>[2x]MNQNLLVTKRDGSTERINLDKIHRVLDWAAEGLHNVSISQVELRSHIQFYDGIKTSDIHETIIKAAADLISRDAPDYQYLAARLAIFHLRKKAYGQFEPPALYDHVVKMVEMGKYDNHLLEDYTEEEFKQMDTFIDHDRDMTFSYAAVKQLEGKYLVQNRVTGEIYESAQFLYILVA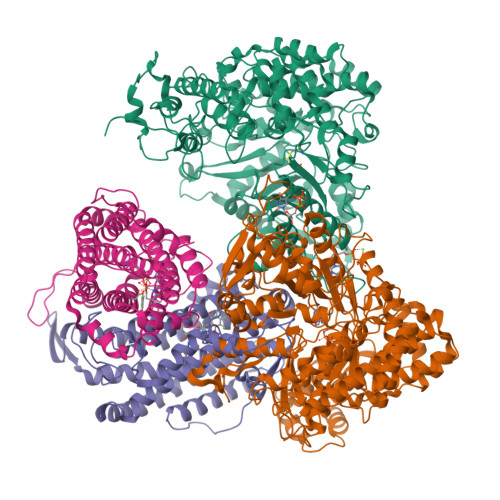ACLFSNYPRETRLQYVKRFYDAVSTFKISLPTPIMSGVRTPTRQFSSCVLIECGDSLDSINATSSAIVKYVSQRAGIGINAGRIRALGSPIRGGEAFHTGCIPFYKHFQTAVKSCSQGGVRGGAATLFYPMWHLEVESLLVLKNNRGVEGNRVRHMDYGVQINKLMYTRLLKGEDITLFSPSDVPGLYDAFFADQEEFERLYTKYEKDDSIRKQRVKAVELFSLMMQERASTGRIYIQNVDHCNTHSPFDPAIAPVRQSNLCLEIALPTKPLNDVNDENGEIALCTLSAFNLGAINNLDELEELAILAVRALDALLDYQDYPIPAAKRGAMGRRTLGIGVINFAYYLAKHGKRYSDGSANNLTHKTFEAIQYYLLKASNELAKEQGACPWFNETTYAKGILPIDTYKKDLDTIANEPLHYDWEALRESIKTHGLRNSTLSALMPSETSSQISNATNGIEPPRGYVSIKASKDGILRQVVPDYEHLHDAYELLWEMPGNDGYLQLVGIMQKFIDQSISANTNYDPSRFPSGKVPMQQLLKDLLTAYKFGVKTLYYQNTRDGAEDAQDDLVPSIQDDGCESGACKI;>[2x]MAYTTFSQTKNDQLKEPMFFGQPVNVARYDQQKYDIFEKLIEKQLSFFWRPEQVDVSRDRIDYQALPEHEKHIFISNLKYQTLLDSIQGRSPNVALLPLISIPELETWVETWAFSETIHSRSXTHIIRNIVNDPSVVFDDIVTNEQIQKRAEGISSYYDELIEMTSYWHLLGEGTHTVNGKTVTVSLRELKKKLYLCLMSVNALEAIRFYVSFACSFAFAERELMEGNAKIIRLIARDEALHLTGTQHMLNLLRSGADDPEMAEIAEECKQECYDLFVQAAQQEKDWADYLFRDGSMIGLNKDILCQYVEYITNIRMQAVGLDLPFQTRSNPIPWINTWLVSDNVQVAPQEVEVSSYLVGQIDSEVDTDDLSNFQL> MLGTGPAAATTAATTSXXXXXXXXXXXXXXSRNEETXXXXXXXXXXXXXXXXXEMSQEEXTRFYDQLNHHIFELVSSSDANERKGGILAIASLIGVEGGNATRIGRFANYLRNLLPSNDPVVMEMASKAIGRLAMAGDTFTAEYVEFEVKRALEWLGADRNEGRRHAAVLVLRELAISVPTFFFQQVQPFFDNIFVAVWDPKQAIREGAVAALRACLILTTQREPKEMQKPQWYRHTFEEAEKGFDETLAKEKGMNRDDRIHGALLILNELVRISSMEGERLREEMEEITQQQLVHDKYCKDLMGFGTKPRHITPFTSFQAVQPQQSNALVGLLGYSSHQGLMGFGTSPSPAKSTXXXXXXXXXXXXXXXXXXXXXXXKCRNSKNSLIQMTILNLLPRLAAFRPSAFTDTQYLQDTMNHVLSCVKKEKERTAAFQALGLLSVAVRSEFKVYLPRVLDIIRAALPPKDFAHKRQKAMQVDATVFTCISMLARAMGPGIQQDIKELLEPMLAVGLSPALTAVLYDLSRQIPQLKKDIQDGLLKMLSLVLMHKPLRHPGMPKGLAHQLASPGLTTLPEASDVGSITLALRTLGSFEFEGHSLTQFVRHCADHFLNSEHKEIRMEAARTCSRLLTPSIHLISGHAHVVSQTAVQVVADVLSKLLVVGITDPDPDIRYCVLASLDERFDAHLAQAENLQALFVALNDQVFEIRELAICTVGRLSSMNPAFVMPFLRKMLIQILTELEHSGIGRIKEQSARMLGHLVSNAPRLIRPYMEPILKALILKLKDPDPDPNPGVINNVLATIGELAQVSGLEMRKWVDELFIIIMDMLQDSSLLAKRQVALWTLGQLVASTGYVVEPYRKYPTLLEVLLNFLKTEQNQGTRREAIRVLGLLGALDPYKHKVNIGMIDQSRDASAVSLSESKSSQDSSDYSTSEMLVNMGNLPLDEFYPAVSMVALMRIFRDQSLSHHHTMVVQAITFIFKSLGLKCVQFLPQVMPTFLNVIRVCDGAIREFLFQQLGMLVSFVKSHIRPYMDEIVTLMREFWVMNTSIQSTIILLIEQIVVALGGEFKLYLPQLIPHMLRVFMHDNSPGRIVSIKLLAAIQLFGANLDDYLHLLLPPIVKLFDAPEAPLPSRKAALETVDRLTESLDFTDYASRIIHPIVRTLDQSPELRSTAMDTLSSLVFQLGKKYQIFIPMVNKVLVRHRINHQRYDVLICRIVKGYTLADEEEDPLIYQHRMLRSGQGDALASGPVETGPMKKLHVSTINLQKAWGAARRVSKDDWLEWLRRLSLELLKDSSSPSLRSCWALAQAYNPMARDLFNAAFVSCWSELNEDQQDELIRSIELALTSQDIAEVTQTLLNLAEFMEHSDKGPLPLRDDNGIVLLGERAAKCRAYAKALHYKELEFQKGPTPAILESLISINNKLQQPEAAAGVLEYAMKHFGELEIQATWYEKLHEWEDPLVAYDKKMDTNKDDPELMLGRMRCLEALGEWGQLHQQCCEKWTLVNDETQAKMARMAAAAAWGLGQWDSMEEYTCMIPRDTHDGAFYRAVLALHQDLFSLAQQCIDKARDLLDAELTAMAGESYSRAYGAMVSCHMLSELEEVI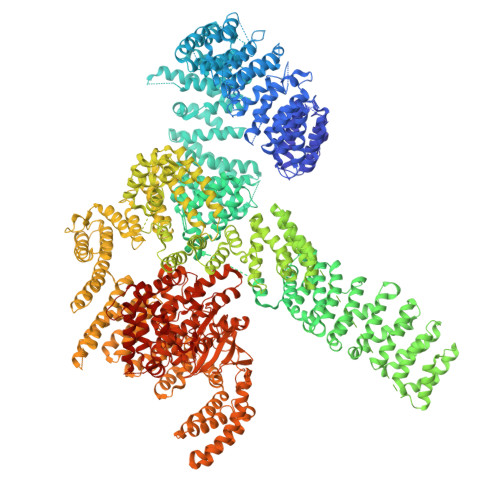QYKLVPERREIIRQIWWERLQGCQRIVEDWQKILMVRSLVVSPHEDMRTWLKYASLCGKSGRLALAHKTLVLLLGVDPSRQLDHPLPTVHPQVTYAYMKNMWKSARKIDAFQHMQHFVQTMQQQAQHAIATEDQQHKQELHKLMARCFLKLGEWQLNLQGINESTIPKVLQYYSAATEHDRSWYKAWHAWAVMNFEAVLHYKHQNQARDEKKKLRHASGANITNATTAATTAATATTTASTEGSNSESEAESTENSPTPSPLQKKVTEDLSKTLLMYTVPAVQGFFRSISLSRGNNLQDTLRVLTLWFDYGHWPDVNEALVEGVKAIQIDTWLQVIPQLIARIDTPRPLVGRLIHQLLTDIGRYHPQALIYPLTVASKSTTTARHNAANKILKNMCEHSNTLVQQAMMVSEELIRVAILWHEMWHEGLEEASRLYFGERNVKGMFEVLEPLHAMMERGPQTLKETSFNQAYGRDLMEAQEWCRKYMKSGNVKDLTQAWDLYYHVFRRISKQLPQLTSLELQYVSPKLLMCRDLELAVPGTYDPNQPIIRIQSIAPSLQVITSKQRPRKLTLMGSNGHEFVFLLKGHEDLRQDERVMQLFGLVNTLLANDPTSLRKNLSIQRYAVIPLSTNSGLIGWVPHCDTLHALIRDYREKKKILLNIEHRIMLRMAPDYDHLTLMQKVEVFEHAVNNTAGDDLAKLLWLKSPSSEVWFDRRTNYTRSLAVMSMVGYILGLGDRHPSNLMLDRLSGKILHIDFGDCFEVAMTREKFPEKIPFRLTRMLTNAMEVTGLDGNYRITCHTVMEVLREHKDSVMAVLEAFVYDPLLNWRLMDTNTKGNKRSRTRTDSYSAGQSVEILDGVELGEPAHKKTGTTVPESIHSFIGDGLVKPEALNKKAIQIINRVRDKLTGRDFSHDDTLDVPTQVELLIKQATSHENLCQCYIGWCPFW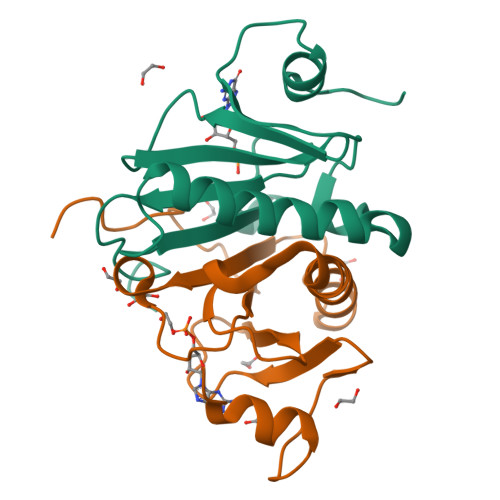>[8x]MAEETIFSKIIRREIPSDIVYQDDLVTAFRDISPQAPTHILIIPNILIPTVNDVSAEHEQALGRMITVAAKIAEQEGIAEDGYRLIMNTNRHGGQEVYHIHMHLLGGRPLGPMLAHKGL> SLYKMSSINADFAFNLYRRFTVETPDKNIFFSPVSISAALVMLSFGACCSTQTEIVETLGFNLTDTPMVEIQHGFQHLICSLNFPKKEL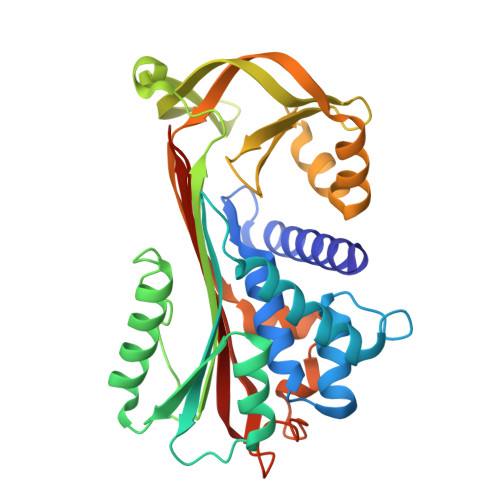ELQIGNALFIGKHLKPLAKFLNDVKTLYETEVFSTDFSNISAAKQEINSHVEMQTKGKVVGLIQDLKPNTIMVLVNYIHFKAQWANPFDPSKTEDSSSFLIDKTTTVQVPMMHQMEQYYHLVDMELNCTVLQMDYSKNALALFVLPKEGQMESVEAAMSSKTLKKWNRLLQKGWVDLFVPKFSISATYDLGATLLKMGIQHAYSENADFSGLTEDNGLKLSNAAHKAVLHIGEKGTEAAGAMFLEAIPR Clomifene | C26 H28 Cl N O | 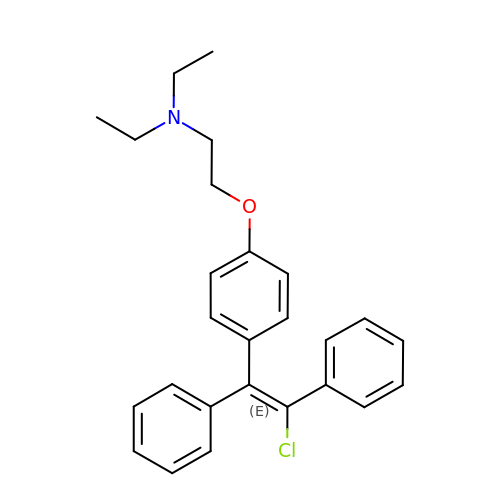GKIRPKYJQBWNGO-OCEACIFDSA-N> SLTHRKFGGSGGSPFSGSGLSSIAVRSGSYLDAIIIDGVHHGGSGGNLSPTFTFGSGEYISNMTIRSGDYIDNI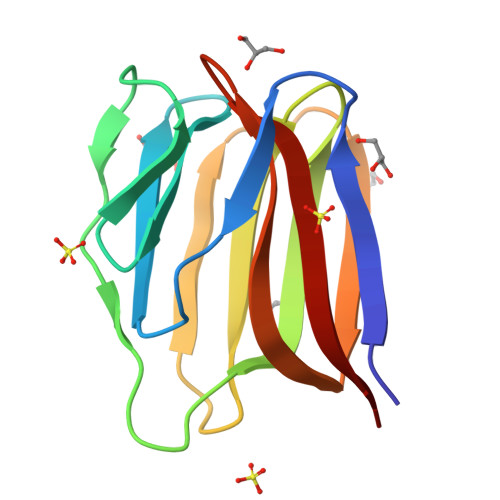SFETNMGRRFGPYGGSGGSANTLSNVKVIQINGSAGDYLDSLDIYYEQY> MIAMDIREIGLRLVGEAIKAADPYRAVLNAVKVSDDKIIVQGKEFEIKGKVYVIALGKAACEMARAIEDILDVEDGVAVTKYGYGKELKRIKVIEAGHPIPDEKSILGAKEALSILNRARENDIVFILISGGGSALFELPEEGISLEDLKLTTDLLLKSGAKIHEINTVRKHISKVKGGKLAKMIKGTGIVLIISDVVGDNLEAIASGPTVKDPTTFEDAKRILELYDIWEKVPESVRLHIERGLRGEVEETLKEDLPNVHNFLIASNSISCEAIAREAQRLGFKAYIMTTTLEGEAKDAGLFIGSIVQEIAERGRPFEPPVVLVFGGETTVTIEGKGGKGGPNQEIALSATRKISDLEALI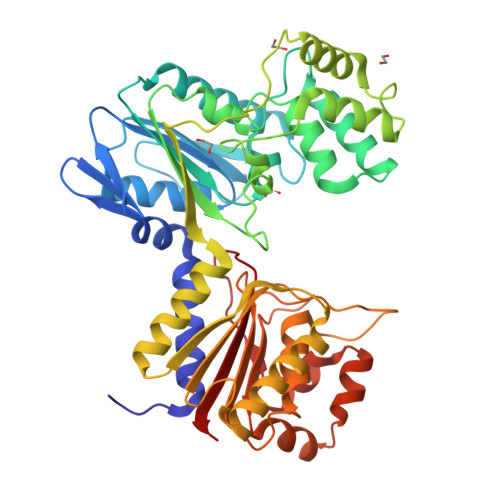VAFDTDGTDGPTDAAGGIVDGTTYKKLREKGIDVEKVLKEHNSYEALKKVGGLLFTGPTGTNVNSIVIAIVTSKRGRT> ERPNCLS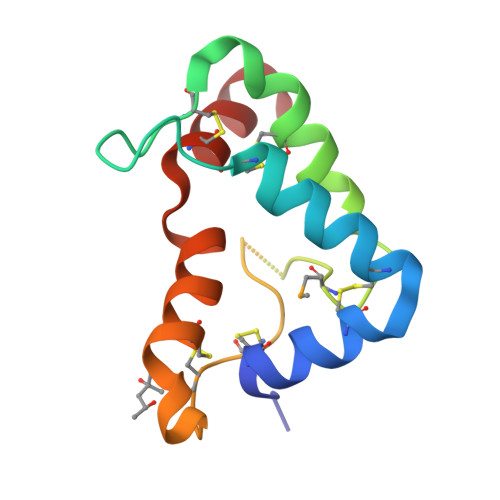LQDSCKTNYICRSRLADFFTNCQPESRSVSNCLKENYADCLLAYSGLIGTVMTPNYVDSSSLSVAPWCDCSNSGNDLEDCLKFLNFFKDNTCLKNAIQAFG>MGPVWRKHYITYRINNYTPDMNREDVDYAIRKAFQVWSNVTPLKFSKINTGMADILVVFARGAHGDDHAFDGKGGILAHAFGPGSGIGGDAHFDEDEFWTTHSGGTNLFLTAVHEIGHSLGLGHSSDPKAVMFP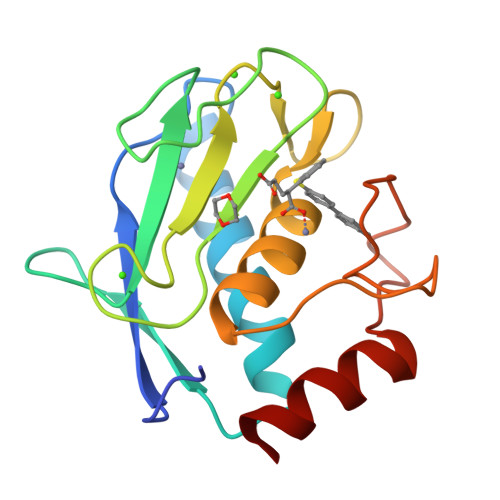TYAYVDINTFRLSADDIRGIQSLYG[4x]>MATSASSHLNKGIKQVYMALPQGDKVQAMYIWIDGTGEGLRCKTRTLDSEPKCIEELPEWNFDGSSTFQSEGSNSDMYLVPAAMFRDPFRKDPNKLVFCEVFKYNRKPAETNL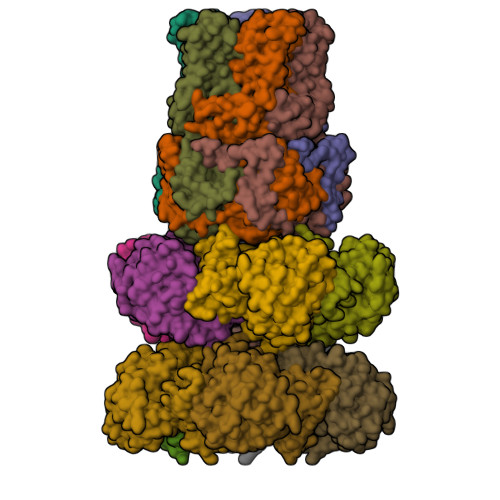RHTCKRIMDMVSNQRPWFGMEQEYTLMGTDGHPFGWPSNGFPGPQGPYYCGVGADKAYGRDIVEAHYRACLYAGIKIGGTNAEVMPAQWEFQIGPCEGIDMGDHLWVARFILHRVCEDFGVIATFDPKPIPGNWNGAGCHTNFSTKAMREENGLKYIEEAIEKLSKRHQYHIRAYDPKGGLDNARRLTGFHETSNINDFSAGVANRGASIRIPRTVGQEKKGYFEDRRPSANCDPFAVTEALIRTCLLNETGDEPFQYKN[10x];>[5x]MTVTYTARVAKARFGGFSKLLLLWRGSIYKLLWRELLCFLGLFMALSAAYRFVLTEEQKRYFEKLVLYCDRYASLIPVSFVLGFYVTLVVHRWWNQYLSMPLTDALMCVVVGTVHGHDERGRLYRRTLMRYAGLSGVLILRSVSTAVFKRFPTIDHVVEAGFMTREERKKFENLNSSYNKYWVPCVWFCNLAAQARREGRIRDNGAFKLLLEELNVFRSKCGMLFHYDWISVPLVYTQVVTIAVYSYFLACLIGRQFLDPAQGYKDHDLDLCVPIFTLLQFFFYAGWLKVAEQLINPFGEDDDDFETNFLIDRCFQVSMLAVDEMYDDLAMLEKDLYWDAAEARAPYTAATAFLMQQPSFQGSTFDITLAKEDMQFQRQDGLEAPLNEAHGDFLQRLLPVGTGMGTGGLL> MGSSHHHHHHSSGRENLYFQGMATITLERDGLQLVGTREEPFGEIYDMAIIFHGFTANRNTSLLREIANSLRDENIASVRFDFNGHGDSDGKFENMTVLNEIEDANAILNYVKTDPHVRNIYLVGHAQGGVVASMLAGLYPDLIKKVVLLAPAATLKGDALEGNTQGVTYNPDHIPDRLPFKDLTLGGFYLRIAQQLPIYEVSAQFTKPVCLIHGTDDTVV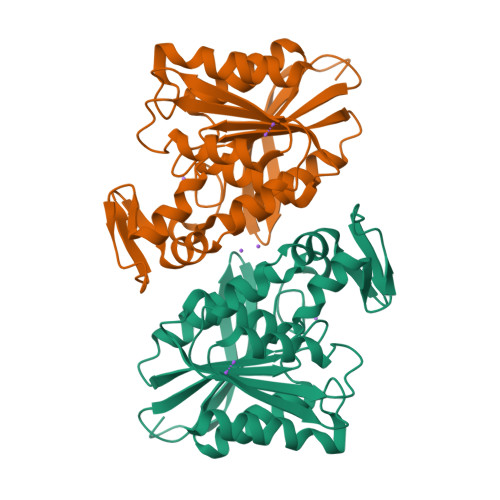SPNASKKYDQIYQNSTLHLIEGADHCFSDSYQKNAVNLTTDFLQNNNAF> MALDRPDRSGAVRVSAPARLSFTLISLDGSSLRRNGIAAMAVDRPGLTAEVREAADGIVAVTGTAEETARELAAALEALRKLWDGPAARVDVLEALPQHSGFGSKTSTLLAVGHAYGRLCGVEPDLRELARTLGRGRVSGASTGLSAYGGFLVDGGHVNPPDFAEAPQKYLRPSRFAQQVAPPKPVVRLDFPDWPVLVLLTHGRHLGGQEELEWFHSVAPIPAEESWRTSHLVFMGLAPAVLEQDFDAFCAAVNEITFTGHFKQAQIAFQGDAVADVLEAGRAAPSVDAIALSVTGPACFAFTKRPEDAERWAWELKNRGLIRDFWFTRANNQGLATTVVS

In the specific case of formycin, the enzyme ForT catalyses C-C bond formation between 4-amino-1H-pyrazole-3,5-dicarboxylate (APDA) and PRPP, in a reaction that is driven by the elimination of CO2 and inorganic pyrophosphate (PPi). ForT catalyses C-C bond formation in formycin A biosynthesis, and we have previously determined its structure complexed to PRPP. This structure establishes that ForT is a member of the GHMP kinase superfamily. ITC measurements show that APDA binds to ForT only in the presence of PRPP, suggesting that the reaction likely follows an ordered bi-bi kinetic mechanism in which PRPP binds first and creates the binding site for APDA. Glu211 is essential for catalysis, and we suggest it acts as a general base to make APDA sufficiently nucleophilic.

In carrying out our preliminary analysis of functionally important active site residues, we discovered that the T138V variant expressed, purified and crystallized more readily than the WT enzyme. Bound PRPP and APDA were easily placed in clear difference electron density in the active site. In our structure, the Mg2+ ion is coordinated in a distorted octahedron to both hydroxyl groups of the ribose, two oxygens in the pyrophosphate moiety and two water molecules (O-Mg2+ distances of 2.0–2.2 Å). The interactions of PRPP with the T138V variant, which are dominated by the 5′-phosphate and the pyrophosphate, are essentially unchanged from those in the WT ForT/PRPP binary complex, and the phosphate moieties are found in almost identical positions in the two structures. Compared to the binary complex, the ribose ring in the T138V ternary complex rotates to create the APDA-binding pocket, a movement that is accomplished merely by changes in the torsion angles connecting the ribose ring to the fixed phosphates at each end of PRPP; akin to a seat of a child's swing linked at both ends to a rigid frame. The planes of the APDA and ribose ring are approximately parallel but do not overlap, thereby positioning the π-system of the pyrazole for nucleophilic attack at C1 of PRPP, and the Val138 side chain adopts the same position and conformation as that seen for Thr138 in the WT ForT/PRPP binary complex. For example, one of the carboxylate groups hydrogen bonds to the backbone NH and side chain of Ser174, which orders residues 172–179 of the protein in the T138V/APDA/MgPRPP ternary complex and positions the adjacent pyrazole carbon 4.6 Å from C1 of PRPP. The other carboxylate of APDA hydrogen bonds to the side chains of Ser21 and Gln266, as well as two water molecules that form a network with the side chain of Glu211. The Leu24 side chain is stacked against one face of the aromatic pyrazole ring. Of course, that the T138V variant is active, albeit with a 40-fold reduction in kcat, poses the question as to why we are able to trap the T138V/APDA/MgPRPP ternary complex.> MRFKKHVVQHEETMQAIAQRYYGDVSYWIDLVEHNNLKYPYLVETDEEKMKDPERLASTGDTLIIPIESDLTDVSAKEINSRDKDVLVELALGRDLNITADEKYFNEHGTSDNILAFSTNGNGDLDTVKGIDNMKQQLQARLLTPRGSLMLHPNYGSDLHNLFGLNIPEQATLIEMEVLRTLTSDNRVKSANLIDWKIQGNVYSGQFSVEIKSVEESINFVLGQDEEGIFALFE;>MKTRKLTNILSKLIDKTMAGTSKITDFTPGSASRSLLEAVSLEIEQFYILTKENIDWGIQEGIIEAFDFQKRQSKRAYGDVTIQFYQPLDMRMYIPAGTTFTSTRQEYPQQFETLVDYYAEPDSTEIVVEVYCKETGVAGNVPEGTINTIASGSSLIRSVNNEYSFNTGTKEESQEDFKRRFHSFVESRGRATNKSVRYGALQIPDVEGVYVYEETGHITVFAHDRNGNLSDTLKEDIIDALQDYRPSGIMLDVTGVEKEEVNVSATVTISNKSRIGDTLQKHIESVIRSYLNNLKTSDDLIITDLIQAIMNIDDVLIYDVSFDNLDENIIVPPQGIIRAGEIKVELK[2x];> MANFLKNLHPLLRRDRNKKDNQDPNFALIDALNEEMNQVEKDAIESKLQSSLKTSTSEYLDKFGDWFGVYRKTDEKDDVYRARIIKYLLLKRGTNNAIIDAIKDYLGRDDIDVSVYEPFTNIFYTNKSHLNGEDHLMGYYYRFAVINVSIGDYFPVEIIDVINEFKPAGVTLYVTYDGASTIRGGAIIKWDDGLPKIETYQEFDRFTGYDDTFYGHINMNQSKDTDNSSSDIFKTNHSLINSLDVLTGSSSVGRQYINYGYVTSYVYNPGMTSSVNQISASTEGRGQEVPTDYYMYTSTKNNNTVELSMQTTSGVSYLYNNFNFRDYMSKYRPQVDLQSDEARRIVSDYIKELSIDYYLSAVIPPDESIEIKLQVYDFSINRWLTVSINNLSFYEKNIGSNIGYIKDYLNSELNMFTRLEINAGKRDSVDIKVNYLDLMFYYYERGIYTIKPYKALIENYLDISRETYVEAFKIASLSNGDIITKTGFQPIGYLKLVGNYENTIPSTINIVAKDTDNNPIESNELDVYNTVENRNLLQSYKGVNTIAREITSTKEFTVSGWAKEIYSTNYLSKVLKPGKVYTLSFDMEITGNDPTLKSYSDNHGIYLYSNTKGIVVNGVKSMERTIGNKVSVTQTFTAPTITDHRLLIYTGRYTSDGKASTPPVFFNTVKITELKLTEGSSKLEYSPAPEDKPNVIEKGIKFNNILTNIQTLSINSDTILKNVTLYYSYYGDSWVELKTLGNISTGETTETNNLIDLYGLQTVDYSNINPMSKVSLRSIWNVKLGELNNQEGSLSNMPNDYFNAVWQDIDKLSDIELGSMRMVKDTEGGVFDGATGEIIKATLFNVGAYTDLDMLAYTLTNYTEPLTLGSSRLISELKEELLTSESFNVDNRIKVIDSIYEELPNTSII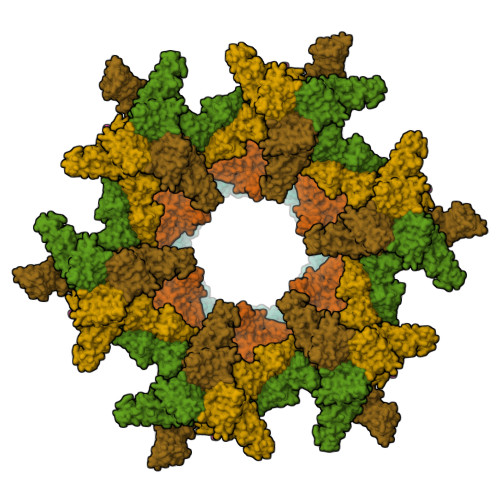KNGFVEREVTGSKYLDYGLYEPIEDGTRYKLIVEGEFKDNIEFISLYNSNPNFNETFIYPSEIINGVAEKEFIAKPSTEDKPRLNTDVRIYIRPYDSTISKVRRVELRKV;>MAINFKGSPYLDRFDPSKDRTKVLFNPDRPLQQAELNEMQSIDQYYLKNLGDAIFKDGDKQSGLGFTLSEDNVLTVNPGYVYINGKIRYYDNDDSVKITGVGKETIGIKLTERIVTPDEDASLLDQTSGVPSYFSKGADRLEEKMSLTVNDPTSATIYTFMDGDLYIQSTNAEMDKINKVLAERTYDESGSYKVNGFELFSEGNAEDDDHVSVVVDAGKAYVKGFKVDKPVSTRISVPKSYDLGTAENESTIFNKSNNSISLANSPVKEIRRVTGQVLIEKERVTRGAQGDGQDFLSNNTAFEIVKVWTETSPGVTTKEYKQGEDFRLTDGQTIDWSPQGQEPSGGTSYYVSYKYNKRMEAGKDYEVTTQGEGLSKKWYINFTPSNGAKPIDQTVVLVDYTYYLARKDSVFINKYGDIAILPGEPNIMRLVTPPLNTDPENLQLGTVTVLPDSDEAVCISFAITRLSMEDLQKVKTRVDNLEYNQAVNALDDGAMEGQNPLTLRSVFSEGFISLDKADITHPDFGIVFSFEDAEATLAYTEAVNQPKIIPGDTTAHIWGRLISAPFTEERTIYQGQASETLNVNPYNIPNKQGVLKLTPSEDNWIDTENVTITEQKTKKVTMKRFWRHNESYYGETEHYLYSNLQLDAGQKWKGETYAYDREHGRTGTLLESGGQRTLEEMIEFIRIRDVSFEVKGLNPNDNNLYLLFDGVRCAITPATGYRKGSEDGTIMTDAKGTAKGKFTIPAGIRCGNREVTLKNANSTSATTYTAQGRKKTAQDIIIRTRVTVNLVDPLAQSFQYDENRTISSLGLYFASKGDKQSNVVIQIRGMGDQGYPNKTIYAETVMNADDIKVSNNASAETRVYFDDPMMAEGGKEYAIVIITENSDYTMWVGTRTKPKIDKPNEVISGNPYLQGVLFSSSNASTWTPHQNSDLKFGIYTSKFNETATIEFEPIKDVSADRIVLMSTYLTPERTGCTWEMKLILDDMASSTTFDQLKWEPIGNYQDLDVLGLARQVKLRATFESNRYISPLMSSSDLTFTTFLTELTGSYVGRAIDMTEAPYNTVRFSYEAFLPKGTKVVPKYSADDGKTWKTFTKSPTTTRANNEFTRYVIDEKVKSSGTNTKLQVRLDLSTENSFLRPRVRRLMVTTRDE[3x]>GSPNSLDQIDLLSTKSFPPCMRQLHKALRENHHLRHGGRMQYGLFLKGIGLTLEQALQFWKQEFIKGKMDPDKFDKGYSFNIRHSFGKEGKRTDYTPFSCLKIILSNPPSQGDYHGCPFRHSDPELLKQKLQSYKISPGGISQILDLVKGTHYQVACQKYFEMIHNVDDCGFSLNHPNQFFCESQR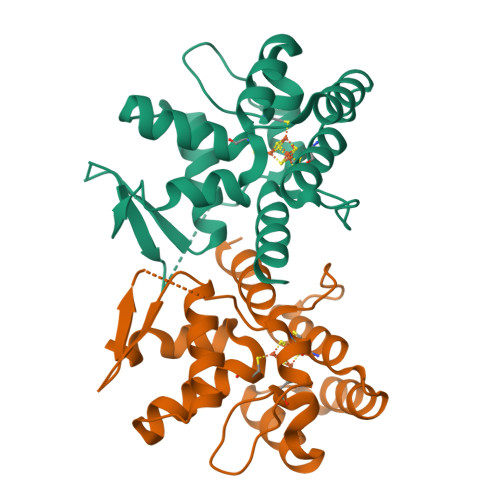ILNGGKDIKKE[4x]>[3x]AVPPPPVNQFLGIYDTKFPNLTKADCLECH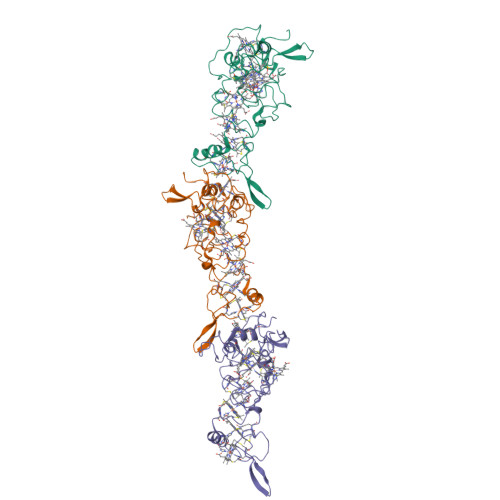VSDTVLVQQHHALINTVTPPASCINTSGTVPPTLATGCHVMVPDGSGGFTFQDFRNCFNCHTQTPHHTSPAAVAKDCKYCHGNFIDNPLDGHYIPTYSASSVTPMPSGRSVTATDGNVVIVQGCEACHQAAPNAIDPKTNTVRPIFSNQDTHHGTGITDCNLCHNTSSNVPIRQCEVCHGVNSLHNIQKDSPNAANLGTVKPGLEDLGWGHIGNNWDCQGCHWSWFGN>[7x]STSAGPTVPDRDNDGIPDSLEVEGYTVDVKNKRTFLSPWISNIHEKKGLTKYKSSPEKWSTASDPYSDFEKVTGRIDKNVSPEARHPLVAAYPIVHVDMENIILSKNEDQSTQNTDSQTRTISKNTSTSRTHTSEVHGNAEVHASFFDIGGSVSAGFSNSNSSTVAIDHSLSLAGERTWAETMGLNTADTARLNANIRYVNTGTAPIYNVLPTTSLVLGKNQTLATIKAKENQLSQILAPNNYYPSKNLAPIALNAQDDFSSTPITMNYNQFLELEKTKQLRLDTDQVYGNIATYNFENGRVRVDTGSNWSEVLPQIQETTARIIFNGKDLNLVERRIAAVNPSDPLETTKPDMTLKEALKIAFGFNEPNGNLQYQGKDITEFDFNFDQQTSQNIKNQLAELNATNIYTVLDKIKLNAKMNILIRDKRFHYDRNNIAVGADESVVKEAHREVINSSTEGLLLNIDKDIRKILSGYIVEIEDTEGLKEVINDRYDMLNISSLRQDGKTFIDFKKYNDKLPLYISNPNYKVNVYAVTKENTIINPSENGDTSTNGIKKILIFSKKGYEIG;> MNIKKEFIKVISMSCLVTAITLSGPVFIPLVQGAGGHGDVGMHVKEKEKNKDENKRKDEERNKTQEEHLKEIMKHIVKIEVKGEEAVKKEAAEKLLEKVPSDVLEMYKAIGGKIYIVDGDITKHISLEALSEDKKKIKDIYGKDALLHEHYVYAKEGYEPVLVIQSSEDYVENTEKALNVYYEIGKILSRDILSKINQPYQKFLDVLNTIKNASDSDGQDLLFTNQLKEHPTDFSVEFLEQNSNEVQEVFAKAFAYYIEPQHRDVLQLYAPEAFNYMDKFNEQEINLSLEELKDQRMLARYEKWEKIKQHYQHWSDSLSEEGRGLLKKLQIPIEPKKDDIIHSLSQEEKELLKRIQIDSSDFLSTEEKEFLKKLQIDIRDSLSEEEKELLNRIQVDSSNPLSEKEKEFLKKLKLDIQPYDINQRLQDTGGLIDSPSINLDVRKQYKRDIQNIDALLHQSIGSTLYNKIYLYENMNINNLTATLGADLVDSTDNTKINRGIFNEFKKNFKYSISSNYMIVDINERPALDNERLKWRIQLSPDTRAGYLENGKLILQRNIGLEIKDVQIIKQSEKEYIRIDAKVVPKSKIDTKIQEAQLNINQEWNKALGLPKYTKLITFNVHNRYASNIVESAYLILNEWKNNIQSDLIKKVTNYLVDGNGRFVFTDITLPNIAEQYTHQDEIYEQVHSKGLYVPESRSILLHGPSKGVELRNDSEGFIHEFGHAVDDYAGYLLDKNQSDLVTNSKKFIDIFKEEGSNLTSYGRTNEAEFFAEAFRLMHSTDHAERLKVQKNAPKTFQFINDQIKFIINS

Following assembly, the anthrax protective antigen (PA) forms an oligomeric translocon that unfolds and translocates either its lethal factor (LF) or edema factor (EF) into the host cell. The toxin functions as a binary A2B toxin, with enzymatic A factors, lethal factor (LF, 91 kDa) and edema factor (EF, 89 kDa), and a cell binding B factor, protective antigen (PA, 83 kDa). Within the endosomal compartment, the acidic environment induces a conformational change in the PA, resulting in the formation of a β-barrel channel that can insert itself into the endosomal membrane. The first α helix and β strand of LF and EF unfold and dock into a deep amphipathic cleft, called the α clamp, which resides at the interface of two PA monomers.

In our PA7-LF channel structure, the LFN (the amino terminal domain of LF) binds two neighboring PA subunits, one denoted as PAN, which binds the N-terminus of LFN, and the other as PAC, which binds the C-terminus of LFN. The cryo-EM density reveals a helix of LFN bound in the α-clamp site, indicating that this site continues to engage the enzymatic factors in the PA channel. This helix of LFN in PA7 α-clamp appears to bind within this site in much the same manner as in the PA8-(LFN)4 pre-channel structure (PDB 3KWV20). However, at 4.6-Å resolution, it is not possible to determine whether hydrogen bonds form within the α-clamp site between LFN β1 and PAN β13. Upon alignment with 3KWV20, nonetheless, β13 in the PA channel and in the PA8-(LFN)4 pre-channel has a highly similar conformation, with the first α-helix (LFN α1) aligning well between the two structures. This alignment indicates that LFN α1 binds within the α-clamp site similarly in both the PA channel and the pre-channel. The catalytic domain of LF is invisible in our EM structure, suggesting that it is flexible. LF α1 is angled downward towards the pore in the α-clamp site, while the amino-terminal end of EF α1 is elevated ~2.9 Å as measured using the carbonyl groups on LF Glu34 and EF Glu24. When bound to the pre-channel, LFN forms numerous stabilizing interactions on its amino and carboxyl terminal subdomains. Upon conversion to the channel conformation, the carboxyl terminal subdomain of LFN destabilizes its interface with PA.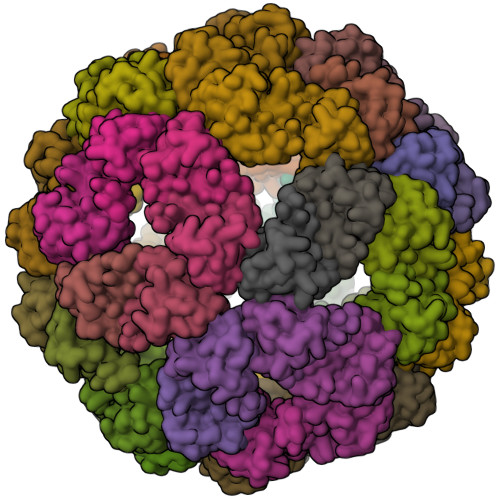>[60x]PDEDLKAELAATEAIWLLRQGRPEEVWKLMQRLYEKGDPALWAVLRALLRSGDEIAILIAWNFMQRI N~6~-(3,4-dimethoxyphenyl)-2-(morpholin-4-yl)-4,5'-bipyrimidine-2',6-diamine 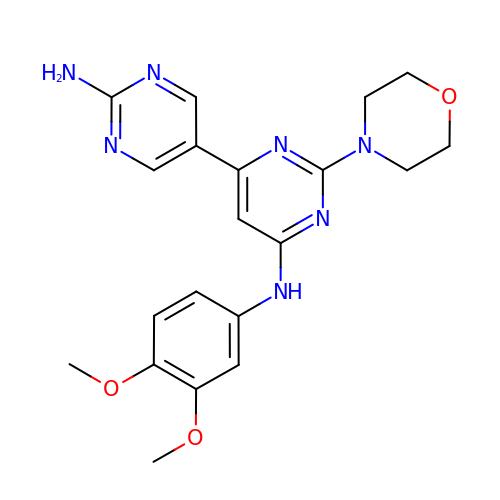| C20 H23 N7 O3 | AAKJGXGPYVKGQA-UHFFFAOYSA-N> MGMTGHHGWGYGQDDGPSHWHKLYPIAQG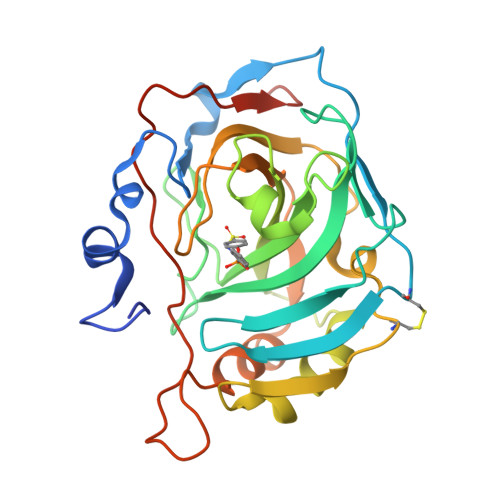DRQSPINIISSQAVYSPSLQPLELSYEACMSLSITNNGHSVQVDFNDSDDRTVVTGGPLEGPYRLKQFHFHWGKKHDVGSEHTVDGKSFPSELHLVHWNAKKYSTFGEAASAPDGLAVVGVFLETGDEHPSMNRLTDALYMVRFKGTKAQFSCFNPKSLLPASRHYWTYPGSLTTPPLSESVTWIVLREPISISERQMGKFRSLLFTSEDDERIHMVNNFRPPQPLKGRVVKASFRALEHHHHHH>[2x]VIVSMIAALANNRVIGLDNKMPWHLPAEL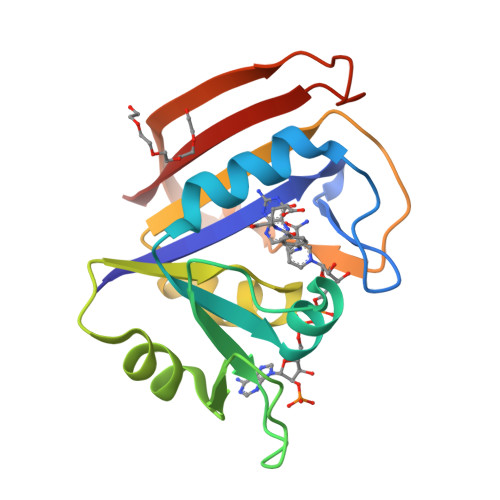QLFKRATLGKPIVMGRNTFESIGRPLPGRLNIVLSRQTDYQPEGVTVVATLEDAVVAAGDVEELMIIGGATIYNQCLAAADRLYLTHIELTTEGDTWFPDYEQYNWQEIEHESYAADDKNPHNYRFSLLERVK>GNSFVGLRVV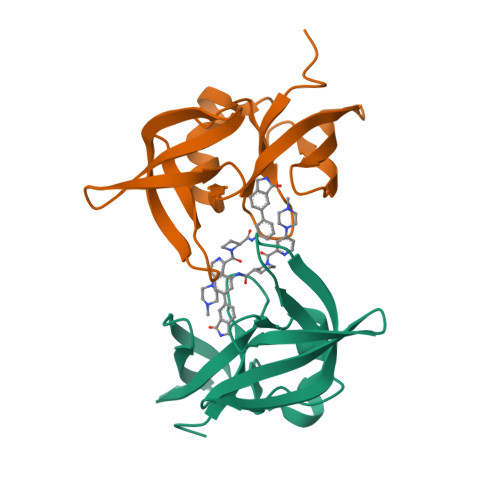AKWSSNGYFYSGKITRDVGAGKYKLLFDDGYECDVLGKDILLCDPIPLDTEVTALSEDEYFSAGVVKGHRKESGELYYSIEKEGQRKWYKRMAVILSLEQGNRLREQYGLGPYE[6x]> F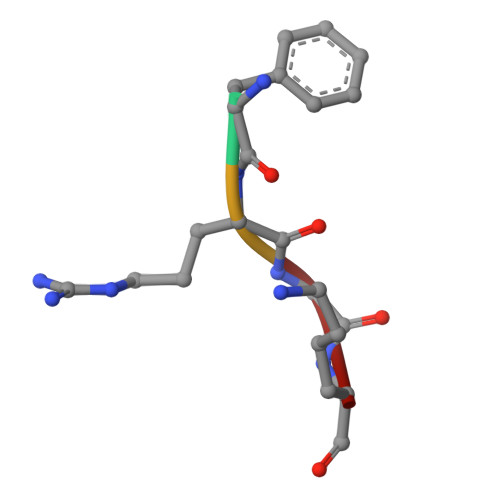RGK> MTVKAMALNTNQLFAYLNRGDIAEFKFSPLFTTLFFPNVATFSTQNIMLDTLDIEEVTMSAFC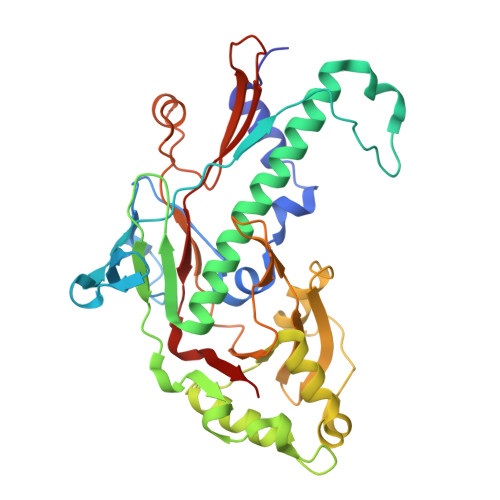SPMVGSQVQRDKGYETSTIKPGYMKPKHEIDPTKTIMRMAGEDPAQLNDPTYRRMRLITGNMRRQINAIKARVEWLAVNAVTTGKNIIEGEGIERYEIDWKIPEKNIIEQADGKKWSEQDKETHYPIYDIELYADQAGCPANVMIMGAEVWRTLRSFKKFRELYDLSRGSESAAELACKNLGEVVSFKGYLGDLALIVYSGKYTDSDGTEKYFLEPDLLVLGNTNNKGLVAYGAIMDQEAVRTGATQNMFYPKNWIEDGDPAIEYVQTHSAPQPVPADIRKFVTVKIA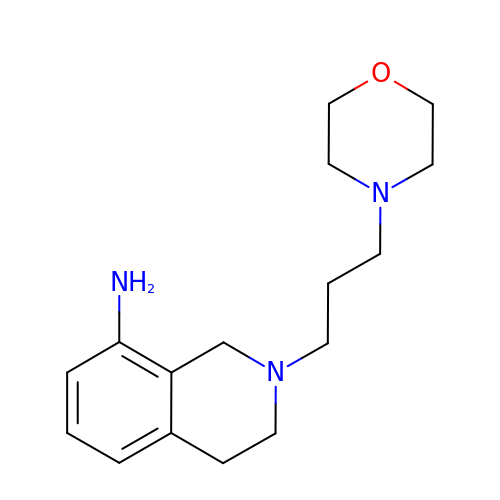2-[3-(morpholin-4-yl)propyl]-1,2,3,4-tetrahydroisoquinolin-8-amine | C16 H25 N3 O | NKWZUNXHZAHVHV-UHFFFAOYSA-N>MPEGPEVALTADILEKYFKGKTLEYIDFISGRYSKSEPEGYDDFIANLPLKVSNVDTKGKFLWFELFDPNDKSNKWYIWNTFGLTGMWSLFEAKYTRAVLSFDNELMAYFSDMRNFGTFKFSNSEKELKRKLNELG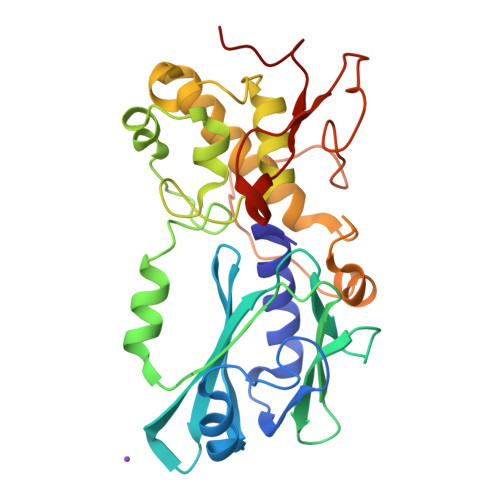PDFLKNDDIDISKIKKYKQPIVALLMDQKKIGSGLGNYLVAEILYRAKIDPHKLGSNLTDQEIENLWYWIKYETKLAYDSNHIGYMVNLENESSKIGRKNYHPNIHPTEKEFDFLVYRKKKDPNGNKVIADKIIGSGKNKRTTYWAPAIQKLE[2x]>MGHHHHHHAENLYFQHMAKIGFIGTGIMGKPMAQNLQKAGHS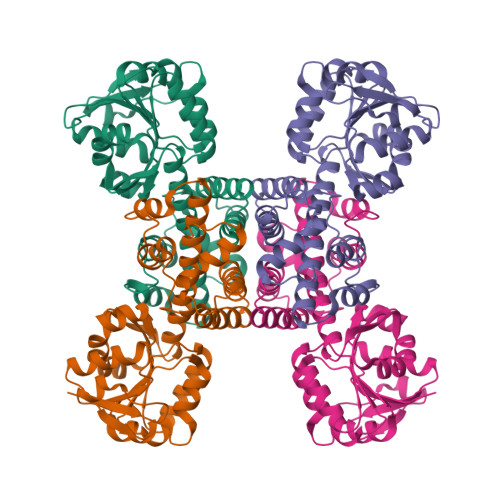LFLSTHHDAAPADLLEAGAIALANPKEVAQEAEFIIVMVPDTPQVEDVLFRKDGIAEGAGPNKVVIDMSSISPTATKGFAEKIKATGAQYLDAPVSGGEVGAKAATLSIMVGGCPNTFERALPLFQAMGKNITRVGGNGDGQTAKVANQIIVALNIQAVAEALLFAARNGADPAKVREALMGGFASSRILEVHGERMVKGTFDPGFRISLHQKDLNLALAGARELNLNLPNTANAQQVFSTCAAIGGSNWDHSALIKGLEHMANFSIRDE[4x]>MRKRRMYLVSWLNSSGVLPNSWNEGRGNRARIFDLENYIRSAEIARRGRIDAFFLADQPQLTPNPKVRPEYPFDPIVLAAAITGRVPDIGGIVTASTSFSLPYTLARQIASVNLLSGGRIGWNAVTTANPAVAANYGAAIATHDNRYERAEEFLEVVHGLWNSWKFPWDEAIGPNPNPFGEVMPINHEGKYFKVAGPLNVPLPPYGPPVVVQAGGSDQGKRLASRFGEIIYAFLGSKPAGRRFVAEARAAARAQGRPEGSTLVLPSFVPLIGSTEAEVKRLVAEYEAGLDPAEQRIEALSKQLGIDLERINVDQVLQEKDFNLPKESATPIGILKSMVDVALDEKLSLRQLALRMRLIAGTPDQVADRLIDWWQDEAADGFVINAPLLPDALEIFVDQVVPILQSRGVFPRSYTES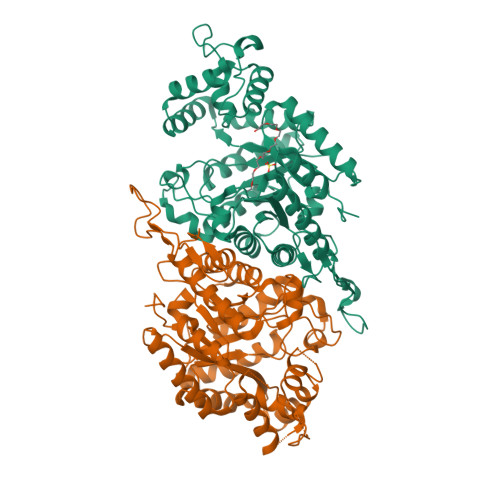TLRERLGLPRNPLG[2x]> MNRRFRYALLPTLALVVAGIAGSAGANDLRGALLAGNCYGCHGPNGDSQGGIPSLSG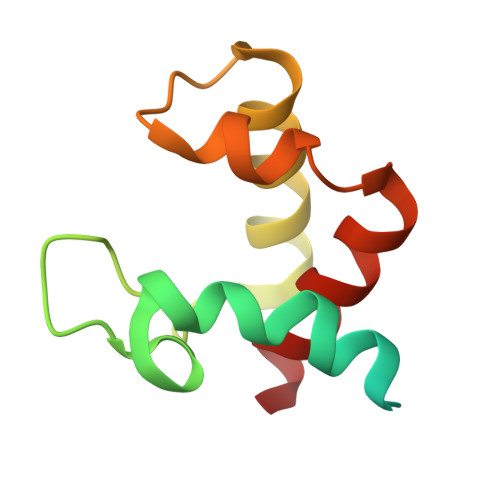LDADQIAETMLAFRSGTRESTVMQRQASGYSEDEIASIAQHIAQH>HMASPQFSQQREEDIYRFLKDNGPQRALVIAQALGMRTAKDVNRDLYRMKSRHLLDMDEQSKAWTIY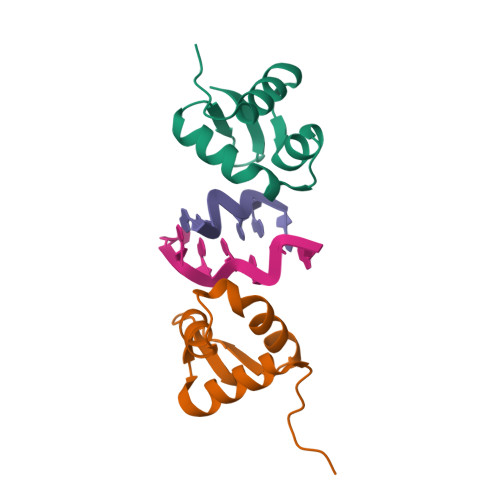RWTIY[2x]> ISGGDAIYSSTGRC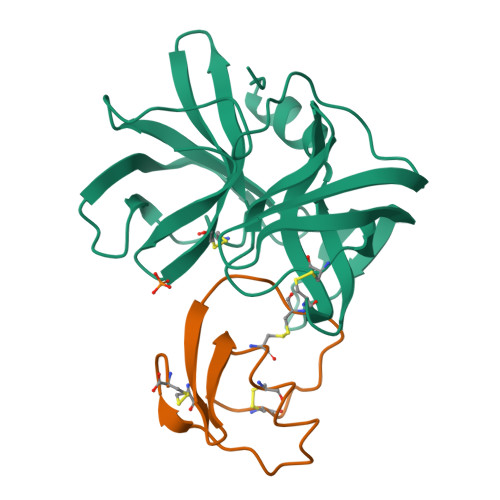SLGFNVRSGSTYYFLTAGHCTDGATTWWANSARTTVLGTTSGSSFPNNDYGIVRYTNTTIPKDGTVGGQDITSAANATVGMAVTRRGSTTGTHSGSVTALNATVNYGGGDVVYGMIRTNVCAEPGDSGGPLYSGTRAIGLTSGGSGNCSSGGTTFFQPVTEALSAYGVSVY;> VDCSEYPKPACTDEYRPLCGSDNKTYGNKCNFCNAVVESNGTLTLSHFGKC>[2x]GPLHMELIQDTSRPPLEYVKGVPLIKYFAEALGPLQSFQARPDDLLISTYPKSGTTWVSQILDMIYQGGDLEKCHRAPIFMRVPFLEFKAPGIPSGMETLKDTPAPRLLKTHLPLALLPQTLLDQKVKVVYVARNAKDVAVSYYHFYHMAKVHPEPGTWDSFLEKFMVGEVSYGSWY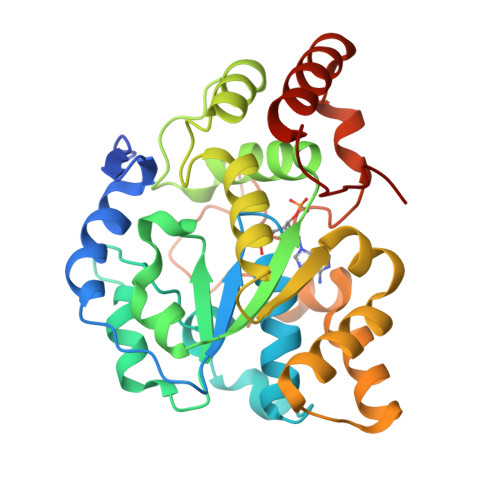QHVQEWWELSRTHPVLYLFYEDMKENPKREIQKILEFVGRSLPEETVDFMVQHTSFKEMKKNPMTNYTTVPQEFMDHSISPFMRKGMAGDWKTTFTVAQNERFDADYAEKMAGCSLSFRSEL ATP-binding cassette transporter B6 (ABCB6), a protein essential for heme biosynthesis in mitochondria, also functions as a heavy metal efflux pump. ATP-binding cassette transporter B6 (ABCB6) is a homodimeric Type IV half-transporter comprising a single transmembrane domain (TMD) and a nucleotide-binding domain (NBD) with an N-terminal extension (TMD0). The TMD is responsible for substrate recognition and translocation, while the NBD is involved in ATP binding and hydrolysis, providing the energy required for substrate transport. In the present study, we determined cryo-electron microscopy (cryo-EM) structures of human ABCB6 in complex with a Cd(II) ion, which is coordinated by two molecules of either GSH or PC2, at resolutions of 3.2 and 3.1 Å, respectively.

However, in the presence of GSH, only Cd(II) significantly increased the ATPase activity of hABCB6core by ~2.4-fold (53 nmol/mg/min) at a saturating concentration of 800 μM, compared with the basal state (22 nmol/mg/min). The structures of hABCB6core in complex with Cd(II) and GSH (or PC2) are shaped like a lassical inward-facing transporter in which the substrate-binding cavity within the TMD region is open towards the cytoplasm. Along with two molecules of GSH (or PC2) with an orientation perpendicular to the membrane, a Cd(II) ion is positioned within the transmembrane pathway of hABCB6core below TM 7 bulge loop (also known as plug). In the Cd(II):GSH structure, the central cysteine of GSH interacts with the Cd(II) ion, functioning as a major coordination site for metal cation binding. By contrast, the glutamate and glycine residues at the N- and C-terminus of GSH, respectively, are not directly involved in Cd(II) binding. Instead, they form a network of hydrogen bonds and van der Waals interactions with residues within the cavity of the transporter, primarily from TM 9, TM 10, and TM 11. These interactions help to neutralize positive charges within the binding cavity, particularly from the arginine clusters (R435, R439, and R552), thus facilitating the stable accommodation of a Cd(II) cation. Consistent with this structural analysis, alanine mutations of the GSH-interacting residues (R435A, R439A, N498A, Q501A, N545A, T549A, and R552A) led to a partial or complete loss of stimulated ATPase activity. Compared with the apo state, binding of Cd(II):GSH at the interface of the two TMDs brings the TM bundles and NBDs toward the center of the transporter. The CASTp program calculated that the cavity volumes of the Cd(II)-bound structures in complex with GSH and PC2 to be approximately 2312 Å3 and 2573 Å3, respectively.

>[2x]APGLRPQSYTLQVHEEDQDVERSQVRSAAQQSTWRDFGRKLRLLSGYLWPRGSPALQLVVLICLGLMGLERALNVLVPIFYRNIVNLLTEKAPWNSLAWTVTSYVFLKFLQGGGTGSTGFVSNLRTFLWIRVQQFTSRRVELLIFSHLHELSLRWHLGRRTGEVLRIADRGTSSVTGLLSYLVFNVIPTLADIIIGIIYFSMFFNAWFGLIVFLCMSLYLTLTIVVTEWRTKFRRAMNTQENATRARAVDSLLNFETVKYYNAESYEVERYREAIIKYQGLEWKSSASLVLLNQTQNLVIGLGLLAGSLLCAYFVTEQKLQVGDYVLFGTYIIQLYMPLNWFGTYYRMIQTNFIDMENMFDLLKEETEVKDLPGAGPLRFQKGRIEFENVHFSYADGRETLQDVSFTVMPGQTLALVGPSGAGKSTILRLLFRFYDISSGCIRIDGQDISQVTQASLRSHIGVVPQDTVLFNDTIADNIRYGRVTAGNDEVEAAAQAAGIHDAIMAFPEGYRTQVGERGLKLSGGEKQRVAIARTILKAPGIILLDEATSALDTSNERAIQASLAKVCANRTTIVVAHRLSTVVNADQILVIKDGCIVERGRHEALLSRGGVYADMWQLQQGQEETSEDTKPQTMER> SYGDNAQNGGGLVIDMPALNRIHSIDSGTRLVDVDAGVSLDQLMKAALPHGLWVPVLPGTRQVTVGGAIGCDIHGKNHHSAGSFGNHVRSMELLTANGEVRHLTPAGPDSDLFWATVGGNGLTGIILRATIEMTPTETAYFIADGDVTGSLDETIAFHSDGSEANYTYSSAWFDAISKPPKLGRAAISRGSLAKLDQLPSKLQKDPLKFDAPQLLTLPDIF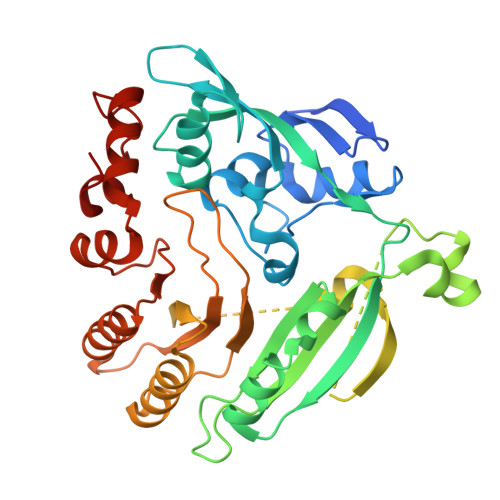PNGLANKFTFMPIGELWYRKSGTYRNKVQNLTQFYHPLDMFGEWNRAYGSAGFLQYQFVVPTEAVEEFKSIIVDIQRSGHYSFLNVFKLFGPGNQAPLSFPIPGWNVCVDFPIKAGLHEFVTELDRRVLEFGGRLYTAKDSRTTAETFHAMYPRIDEWIRIRRSVDPDGVFASDMARRLQLL>[8x]SNAMLDSVASTLQLSELLSLTKAEQSIRLAEINVELEMLSAQERVAWALQNLEGAHAVSSSFGIQAAVMLHLVSKQQADIPVILTDTGYLFPETYQFIDELTKSLNLNLKVYRANESANWQEARYGKLWEQ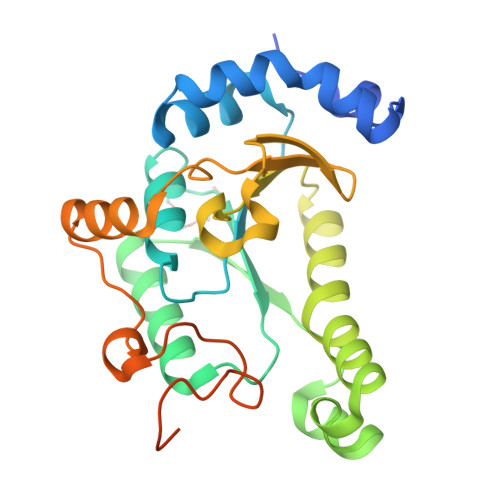GIEGIEKYNKLNKVEPMRRALNELNVKTWFSGLRREQSQSRAGLPILSIQNGVFKFLPVVDWSNKDVHYYLKEHGLSYHPLWEQGYLSVGDTHTTQKWEPGMSEEETRFFGLKRECGLHEEDNEQDGSGI> MKAMHVAQPAVVLASSRGIASFVCEYASPGKATEVRVTVLRQADSQVTEVCA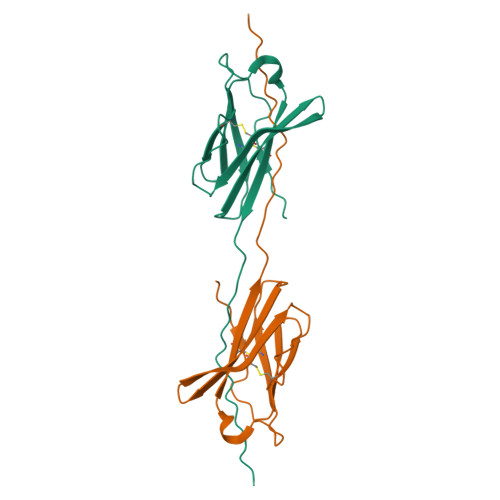ATYMMGNELTFLDDSICTGTSSGNQVNLTIQGLRAMDTGLYICKVELMYPPPYYLGIGNGTQIYVIDPEPSPDSDLVPR D-ORNITHINE | C5 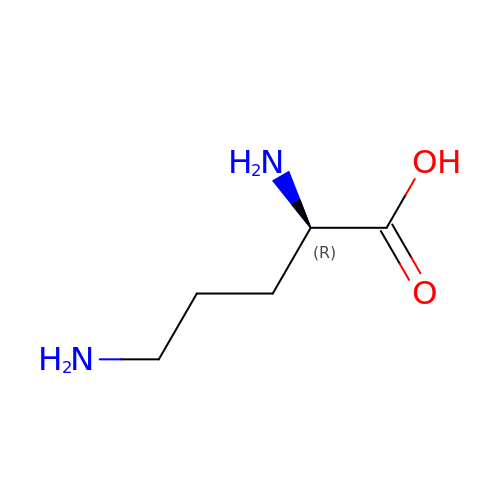H12 N2 O2 | AHLPHDHHMVZTML-SCSAIBSYSA-N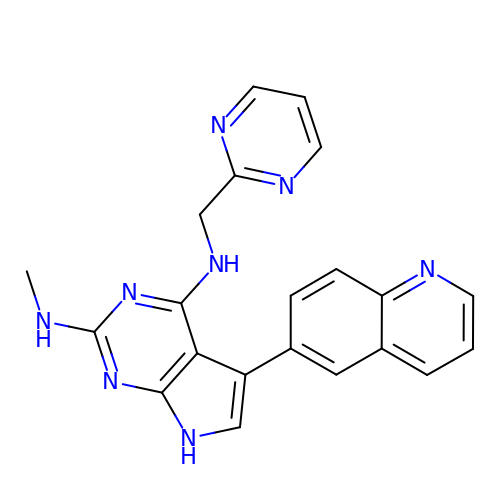N~2~-methyl-N~4~-[(pyrimidin-2-yl)methyl]-5-(quinolin-6-yl)-7H-pyrrolo[2,3-d]pyrimidine-2,4-diamine | C21 H18 N8 | PMWVYONICYRLNY-UHFFFAOYSA-N>[4x]TSEDACQDAEQPTRYETLFQALDRNGDGVVDIGELQEGLRNLGIPLGQDAEEKIF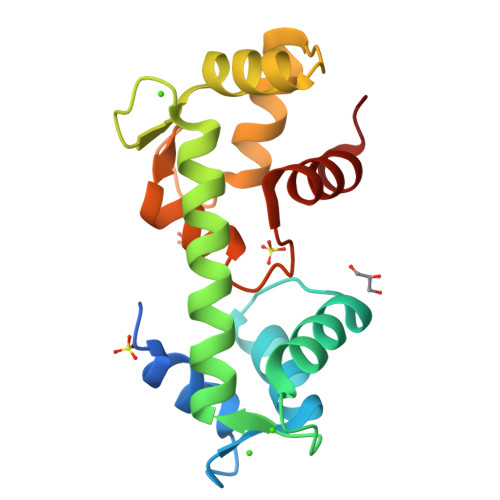TTGDVNKDGKLDFEEFMKYLKDHEKKMKLAFKSLDKNNDGKIEASEIVQSLQTLGLTISEQQAELILQSIDVDGTMTVDWNEWRDYFLFNPVTDIEEIIRFWKHSTGIDI> MADLNWISSALIKERPSADAVLAKAVLAAREQLGLTQLELAGIVGVDRSAISRWKTQGLRVDSKTGELALLLVRVYRALYALFGGQQEDMRHFLRTPNHHLAGEPL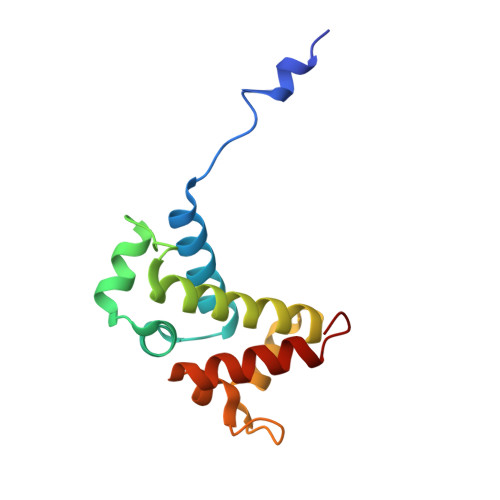ALMGQVQGLVHVLEYLDAIRGKV> MAIIETTTPTEEEAKA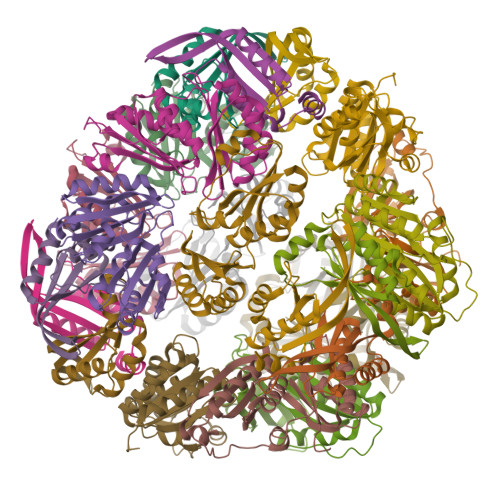IAKKLLENRLIAEAIITPALTKIYRENGEIKSETVTRVTLYTEEENVPKAVTYIKAIHPDPIPPIIVITPTDANPAYKGWVAFET;> MHHHHHHGGSHHWGGDPERPALGILELSSYARGVKVADAALKAAPVKLLKCEPVEPGRALIMLLGEPEDVAKAMIAALDVAGLGSGNLIDYALIPEIHPQLLPFLKEYKKSEPIKDPNKAIIVAEVSTVAAAIEAADVALRLANVELTSMRLAEHIGGRASFTLIGDKEDVEKAARAIRGVAGERLLDLEIIEKPVEALIGNEFF>[2x]MHHHHHHHHGSENLYFQSVKL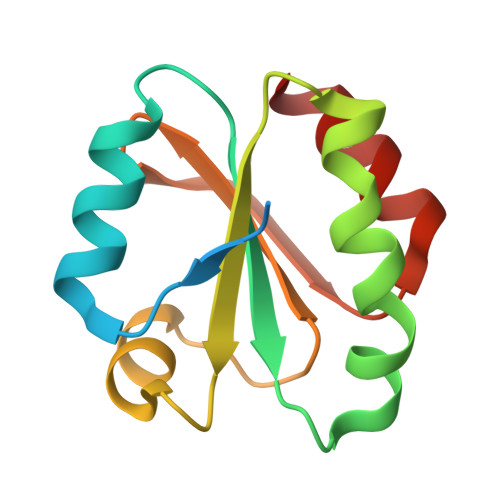IESKEAFQEALAAAGDKLVVVDFSATWCGPCKMIKPFFHSLCDKYSNVVLLEVDVDDCQDVAADCEVKCMPTFQFYKKGQKVGEFSGANKEKLEATITEFA> NSSTASKTYNYVYSSDPSSLNYLAENRAATSDIVANLVDGLLENDQYGNIIPSLAEDWTVSQDGLTYTYKLRKDAKWFTSEGEEYAPVTAQDFVTGLQYAADKKSEALYLVQDSVAGLDDYITGKTSDFSTVGVKALDDQTVQYTLVKPELYWNSKTLATILFPVNADFLKSKGDDFGKADPSSILYNGPFLMKALVSKSAIEYKKNPNYWDAKNVFVDDVKLTYYDGSDQESLERNF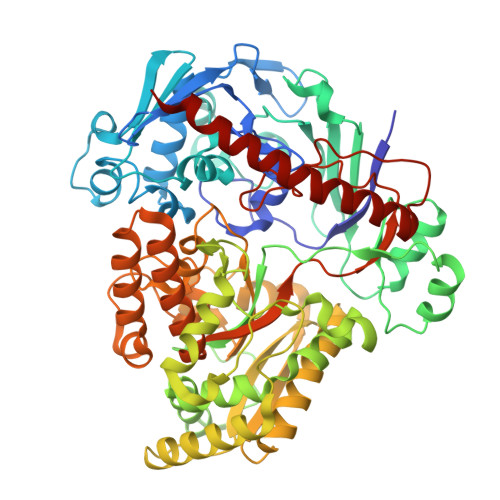TAGAYTTARLFPNSSSYEGIKEKYKNNIIYSMQNSTSYFFNFNLDRKSYNYTSKTSDIEKKSTQEAVLNKNFRQAINFAFDRTSYGAQSEGKEGATKILRNLVVPPNFVSIKGKDFGEVVASKMVNYGKEWQGINFADGQDPYYNPEKAKAKFAEAKKELEAKGVQFPIHLDKTVEVTDKVGIQGVSSIKQSIESVLGSDNVVIDIQQLTSDEFDSSGYFAQTAAQKDYDLYHGGWGPDYQDPSTYLDIFNTNSGGFLQNLGLEPGEANDKAKAVGLDVYTQMLEEANKEQDPAKRYEKYADIQAWLIDSSLVLPSVSRGGTPSLRRTVPFAAAYGLTGTKGVESYKYLKVQDKIVTTDEYAKAREKWLKEKEESNKKAQEELAKHVK>MNDLERLFNPSAIAVVGASKDPSKIGSQILRNLLSYGFKGKVYPINPTADELMGLKCYPKVSDVPDKVDVAVISVPSDKVLGVIDDCGKAGVKFAVVITSGFKEVGNEELEEELVRRAHSYGMRVLGPNIFGYLYAPARLNATFGPKDVLSGNVAFISQSGALGIALMGYTVVENIGISSIVSVGNKADLDDVDLLDFFDKDPNTGVIMIYLEGIAPGRGRMFIDVASRVSLRKPIIVIKAGRTEVGARAAASHTGSIAGSVAIYESAFKQSGILMAKSVEDAFDWTKALSWNPIPEGERLIVLTNGG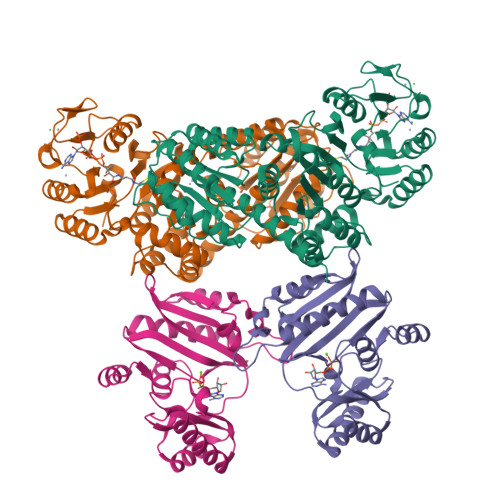GAGVQSTDTFADNGIYLSKPPESLIQEIKKFVPPFASFANPIDITGMAPDDWYYMGTLAALKNPDVDALTVLYCQTAVTTPIGVAKGIVDAIKEAGNSKPVTVGMVGGPEVAEAVSFLNKQRIAAYPTPERASSAMSALYAYARARSYVMKSLAVR[2x];>MSSRDLLLKAKENGRKSLLEHEAKYFISSYGIPVTNIRLAKSEEEAVNFSREIGFPVVLKIVSPQVVHKSDVGGVKVNLRSEEEVRKAYREIIENVKRNVPNAEIEGILVQEFAPPGVELIIGLLRDPQFGPTVMFGLGGVFVELFRDVSFRVAPLSEQDAESMIKEVKAYKLLTGFRGMEPVDIEAIKDALIRAGRIGVENEEIAEMDLNPVIAYPKGIKVVDARIILR[2x]>[2x]MAASTPVVVDIHTHMYPPSYIAMLEKRQTIPLVRTFPQADE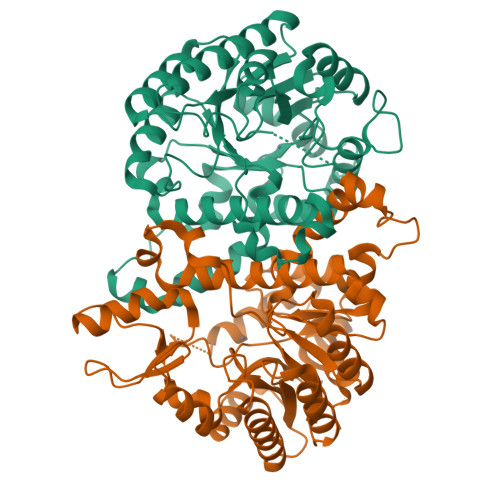PRLILLSSELAALDAALADPAAKLPGRPLSTHFASLAQKMHFMDTNGIRVSVISLANPWFDFLAPDEAPGIADAVNAEFSDMCAQHVGRLFFFAALPLSAPVDAVKASIERVKNLKYCRGIILGTSGLGKGLDDPHLLPVFEAVADAKLLVFLHPHYGLPNEVYGPRSEEYGHVLPLALGFPMETTIAVARMYMAGVFDHVRNLQMLLAHSGGTLPFLAGRIESCIVHDGHLVKTGKVPKDRRTIWTVLKEQIYLDAVIYSEVGLQAAIASSGADRLMFGTNHPFFPPIEEDVQGPWDSSRLNAQAVIKAVGEGSSDAAAVMGLNAVRVLSLKAE>SFGSDVRPAAAQEVVGGGDLGPNVLVFDPSTPDIQGKVDEVFRKQESNQFGTDRYALMFKPGTYNDINAQIGFYTSIAGLGLNPDDTTFNGDVTVDAGWFDGNATQNFWRSAENLALNPVNGTNRWAVSQAAPFRRMHVKGGLNLAPDGYGWASGGYIADSKIDGEVGPYSQQQWYTRDSSVGGWGNGVWNMTFSGVEGAPAQSFPEPPYTTLETTPVSREKPFLYLDGDDYKVFVPAKRTNARGTSWGNGTPEGESLPLDQFYVVKPGATAETINAAVDQGLHLLFTPGVYHVDQPIEIDRANTVALGLGLATIIPDNGVTALKVGDVDGVKVAGLLVDAGPVNSETLVEVGSDGASGDHAANPTSLQDVFVRIGGAGPGKATTSIVVNSNDTIIDHTWVWRADHGEGVGWETNRADYGVHVKGDNVLATGLFVEHFNKYDVQWSGENGKTIFYQNAKAYDAPDQAAIQNGDIKGYAAYKV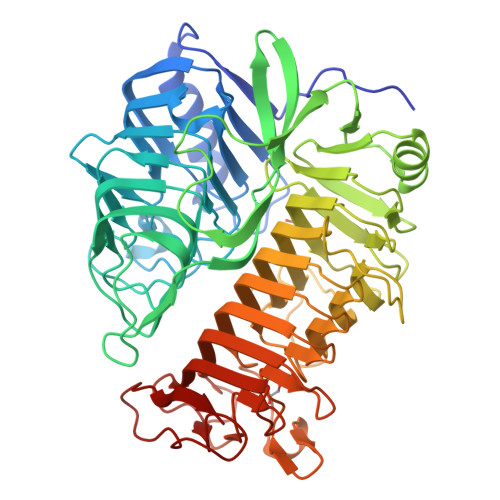DDSVTTHEGWGMGSYCYFNVNPDIRQQHGFQAPVKPGVKFHDLLVVSLGGKGQYEHVINDIGDPTSGDTTIPSQVVSFP[2x]> MNGDETKKVESEYIKKHHRHELVESQCSSTLVKHIKAPLHLVWSIVRRFDEPQKYKPFISRCVVQGKKLEVGSVREVDLKSGLPATKSTEVLEILDDNEHILGIRIVGGDHRLKNYSSTISLHSETIDGKTGTLAIESFVVDVPEGNTKEETCFFVEALIQCN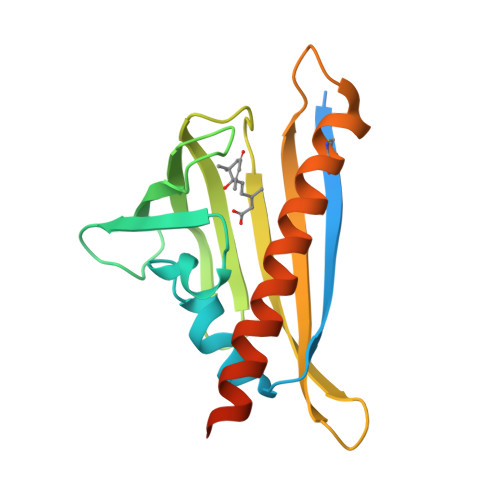LNSLADVTERLQAESMEKKILEHHHHHH>MPVEKDLKTAYKALYDEKEPLKALHLYDEILKGSPTNLTALIFKAACLEKLYFGFSDWHSDATMENAKELLDKALMTAEGRGDRSKIGLVNFRYFVHFFNIKDYELAQSYFKKAKNLGYVDDTLPLWEDRLETKLNKKNKKQKDSTNKHT[3x];> MVTSNVVLVSGEGERFTVDKKIAERSLLLKNYLNDASGDDDDEDDDEIVMPVPNVRSSVLQKVIEWAEHHRDSNFPDEDDDDSRKSAPVDSWDREFLKVDQEMLYEIILAANYLNIKPLLDAGCKVV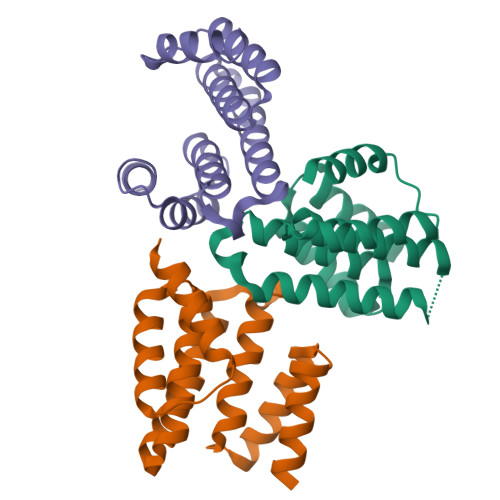AEMI> MKALHFGAGNIGRGFIGKLLADAGIQLTFADVNQVVLDALNARHSYQVHVVGETEQVDTVSGVNAVSSIGDDVVDLIAQVDLVTTAVGPVVLERIAPAIAKGLVKRKEQGNESPLNIIACENMVRGTTQLKGHVMNALPEDAKAWVEEHVGFVDSAVDRIVPPSASATNDPLEVTVETFSEWIVDKTQFKGALPNIPGMELTDNLMAFVERKLFTLNTGHAITAYLGKLAGHQTIRDAILDEKIRAVVKGAMEESGAVLIKRYGFDADKHAAYIQKILGRFENPYLKDDVERVGRQPLRKLS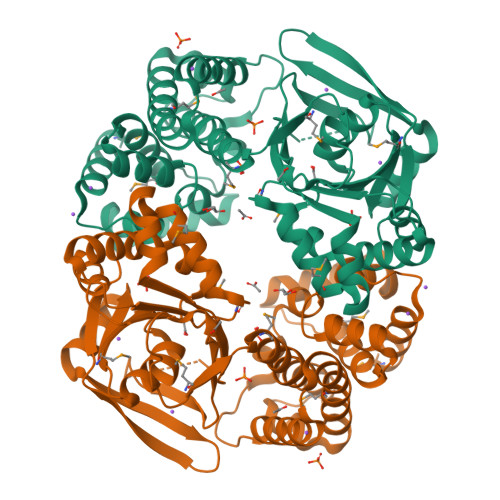AGDRLIKPLLGTLEYSLPHKNLIQGIAGAMHFRSEDDPQAQELAALIADKGPQAALAQISGLDANSEVVSEAVTAYKAMQ>[12x]MAAKQQERTYIMVKPDGVQRGLVSEVIRRFEQRGYKLVALKMKSPD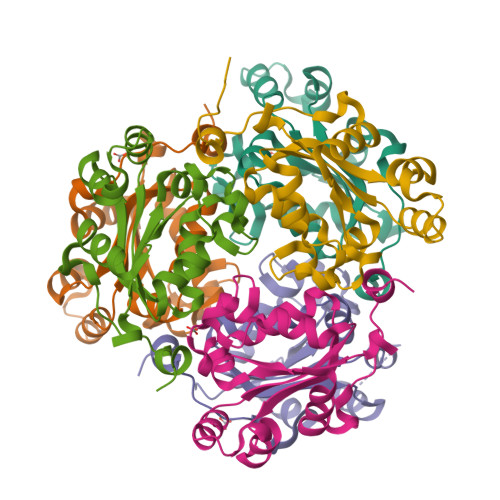ATLLEEHYADLKGKPFFPGLISYMTSGPVVCMVWEGTDVVKQGRRMLGETRPLESNPGTLRGDFCIDVGRNIVHGSDSVESANKEISLWFTPEEICEWTSAQHKWVYEQGENLY N-benzyl-2-[(Z)-iminomethyl]pyrimidine-5-carboxamide | C13 H12 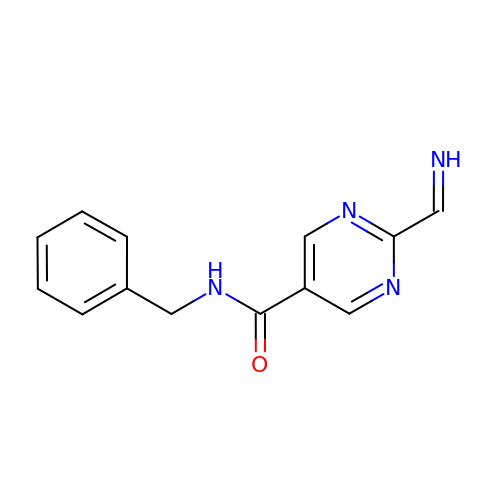N4 O | LOHVEJATQLMRBB-MKMNVTDBSA-N> MQDFQMPKGPAEDTYSTSWTNVNYASDSLESHNLDIYLPKEQKTAYKAIIIIYGSAWFANNAKAMASASIGAPLLKAGFAVISINHRSSMEAIW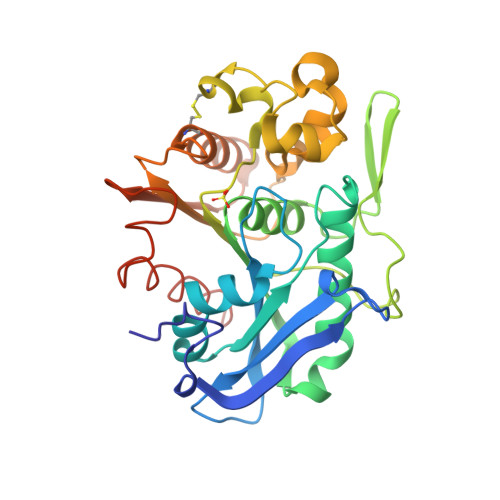PAQIQDVKAAIRYVRSNAAKYNIDPSFIGITGFSSGGHLSAFAGVTNGVKTLTSGDLTVDIEGSLGNYLSTGSHVDAVVDWFGPVDMAHMSNCVAPNDASTPEAVLIGKKDPREEPDWVKLISPINFVDKDDPDILIIHGDADNVVPHCQSVNLKNVYDNAGAKATFISVPGGGHGPGCFDTQYFKDMTDFFTEQSTKLEHHHHHH> MAHVAEWKKKEVEELAKLIKSYPVIALVDVSSMP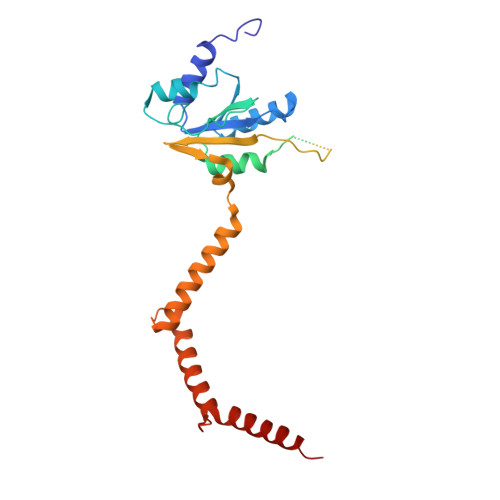AYPLSQMRRLIRENGGLLRVSRNTLIELAIKKAAKELGKPELEKLVEYIDRGAGILVTNMNPFKLYKFLQQNRQPAPAKPGAVVPKDVVVPAGPTPLAPGPIVGQMQALGIPARIEKGKVTIQKDTTVLKAGEVITPELANILNALGIQPLEVGLDVLAVYEDGIVYTPDVLAIDEQEYIDMLQKAYMHAFNLAVNIAYPTPETIEAIIQKAFLNAKTVAIEAGYITKETIQDIIGRAFRAMLLLAQQLP> QEERNQQQDDIEELETKAVGMSNDGRFLKFDIEIGRGSFKTVYKGLDTETTVEVAWCELQERKLTKSERQRFKEEAEMLKGLQHPNIVRFYDSWESTVKGKKCIVLVTELMTSGTLKTYLKRFKVMKIKVLRSWCRQILKGLQFLHTRTPPIIHRDLKCDNIFITGPTGSVKIGDLGLATLKRASFAKSVIGTPEFMAPEMYEEKYDESVDVYAFGMCMLEMATSEYPYSECQNAAQIYRRVTSGVKPASFDKVAIPEVKEIIEGCIRQNKDERYSIKDLLNHAFFQEET

With No Lysine (WNK) kinases are soluble intracelluar serine–threonine kinases noted for their unique active site and their association with familial hyperkalemic hypertension (FHHt). WNKs are the chloride-inhibited protein kinases long anticipated to control the activity of cation chloride cotransporters in response to osmotic stress. WNKs are activated by osmotic stress in cells and are inhibited by chloride. A model for WNK regulation, then, is the presence of a dimer–monomer equilibrium: the dimer is inactive and binds inhibitory ligands; the monomer is autophosphorylation-competent.

Here, we present crystallographic data that the osmolyte PEG400, when applied to crystals of uWNK1, induces de-dimerization and conformational changes. Remarkably, PEG400 induced a space group change from P1 to P21. Together with the space group change, uWNK1/SA in PEG400 monomerizes. No PEG400 was observed in uWNK1/SA/PEG400. Prominent changes occur in helix C and β5, with the largest change occurring in the Activation Loop (including the preceding 3/10 chloride-binding helix). Furthermore, PEG400 induces a large rotation in the 3/10 helix and neighboring helix C. The change in the 3/10 helix eliminates the chloride-binding site and gives rise to big conformational changes at K375 and E388 in the Activation Loop. The water network at the dimer interface, CWN2, is completely lost in PEG400 with the loss of the interface. Data presented here show that PEG400 applied to crystals of WNK1 rearranged and eliminated the AL-CL Cluster and the associated network of water molecules, CWN1. Comparison of the water structure in the inactive dimer versus the PEG400-induced conformation suggests that water functions as an inhibitor, binding and stabilizing an inactive WNK configuration.>IITPALISALKTSFQKHFQDALATAPSTYLQVATVIPSTTASNTYGWLGQFPKLREWIGQRVIKDMAAQGYQITNKLFESTVGVKRTDIEDDNLGVYGPLMQEMGRAAGAHPDELVFALLKAGNANLCYDGQNFFDTDHPVYPNVDGTGTATTVSNLFAPAADPGAAWYLLDTSRSLKPLIYQERMKPSFTSMTKEDDEQVFMADEYRYGVRSRCNVGFGFWQLAAMSTEELNQVNFEKVYDAMRNQKADGGRPLDIRPNLLVVPTTLRSKAKEVVGVQRLANGADNPNFELVQVLDTAWLN[7x]

Bacteriophage Casadabanvirus JBD30, from the order Caudoviricetes, is a temperate phage that infects the bacterium Pseudomonas aeruginosa. The virion of bacteriophage JBD30 is composed of an icosahedral capsid, long flexible non-contractile tail, and a baseplate. Using its baseplate, JBD30 attaches to Pseudomonas aeruginosa via the bacterial type IV pilus, whose subsequent retraction brings the phage to the bacterial cell surface.

The heads of tailed phages assemble as procapsids. The sample of JBD30 used for the collection of electron micrographs contained a fraction of procapsids, which enabled their structure determination. The procapsid of JBD30 has thicker walls and is more spherical than the mature capsid. The hexamers, built from the major capsid proteins, in the procapsid are compressed and skewed, as was observed in the procapsids of other phages. The diameter of the procapsid is 556 Å, which is 6.8% smaller than the diameter of the mature capsid (596 Å). Pores along the central axes of the pentamers (15 Å diameter) and hexamers (13 Å diameter) are wide enough to enable the escape of scaffolding proteins from the procapsid. No decoration proteins are present at the procapsid surface, since the binding sites for the minor capsid proteins are not formed because the arrangement of major capsid proteins differs from that of the mature head. The expansion of the procapsid into a mature capsid is enabled by conformational changes to the major capsid protein. During capsid maturation the N-terminal arm (residues 6–25), which is an α-helix in the procapsid, extends, unfolds, and rotates ~40° anti-clockwise.> GSGASQFFKDNCNRTTASLVEGVELTKYISDINNNTDGMYVVSSTGGVWRISRAKDYPDNVMTAEMRKIAMAAVLSGMRVNMCASPASSPNVIWAIELE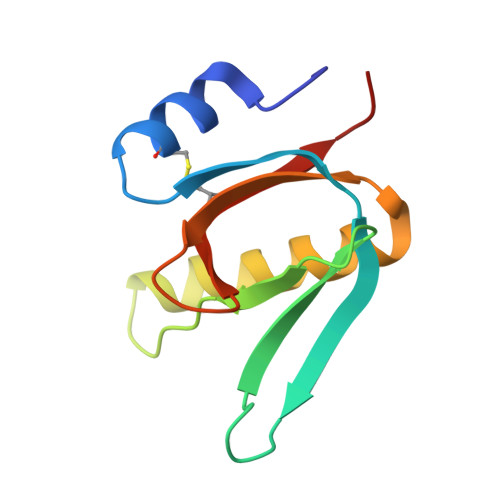AEGS>[2x]MDKIYIHDMEFYGYHGVFPEENKLGQRFK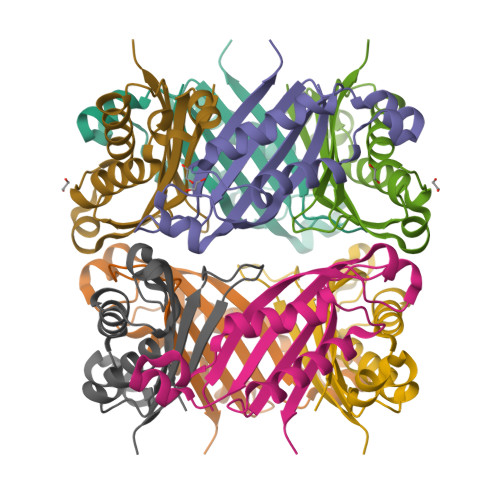VDLTVELDLKRAGESDDLEHSVNYGELFELCRKVVEDRTYKLVESIAENIATDILKQYESISRCTIKVIKPDPPIPGHYRAVAVEITRERP>MLESKLKAPVFTATTQGDHYGEFVLEPLERGFGVTLGNPLRRILLSSIPGTAVTSVYIEDVLHEFSTIPGVKEDVVEIILNLKELVVRFLDPKMASTTLILRAEGPKEVRAGDFTPSADVEIMNPDLHIATLEEGGKLYMEVRVDRGVGYVPAERHGIKDRINAIPVDAIFSPVRRVAFQVEDTRLGQRTDLDKLTLRIWTDGSVTPLEALNQAVAILKEHLNYFANPEASLLPTPEVSKGEKRESAEEDLDLPLEELGLSTRVLHSLKEEGIESVRALLALNLKDLRNIPGIGERSLEEIRQALAKKGFTLKE[4x];>MEIKRFGRIREVIPLPPLTEIQVESYKKALQADVPPEKRENVGIQAAFKETFPIEEGDKGKGGLVLDFLEYRIGDPPFSQDECREKDLTYQAPLYARLQLIHKDTGLIKEDEVFLGHLPLMTEDGSFIINGADRVIVSQIHRSPGVYFTPDPARPGRYIASIIPLPKRGPWIDLEVEASGVVTMKVNKRKFPLVLLLRVLGYDQETLVRELSAYGDLVQGLLDEAVLAMRPEEAMVRLFTLLRPGDPPKKDKALAYLFGLLADPKRYDLGEAGRYKAEEKLGVGLSGRTLVRFEDGEFKDEVFLPTLRYLFALTAGVPGHEVDDIDHLGNRRIRTVGELMADQFRVGLARLARGVRERMVMGSPDTLTPAKLVNSRPLEAALREFFSRSQLSQFKDETNPLSSLRHKRRISALGPGGLTRERAGFDVRDVHRTHYGRICPVETPEGANIGLITSLAAYARVDALGFIRTPYRRVKNGVVTEEVVYMTASEEDRYTIAQANTPLEGDRIATDRVVARRRGEPVIVAPEEVEFMDVSPKQVFSLNTNLIPFLEHDDANRALMGSNMQTQAVPLIRAQAPVVMTGLEERVVRDSLAALYAEEDGEVVKVDGTRIAVRYEDGRLVHPLRRYARSNQGTAFDQRPRVRVGQRVKKGDLLADGPASEEGFLALGQNVLVAIMPFDGYNFEDAIVISEELLKRDFYTSIHIERYEIEARDTKLGPERITRDIPHLSEAALRDLDEEGIVRIGAEVKPGDILVGRTSFKGEQEPSPEERLLRSIFGEKARDVKDTSLRVPPGEGGIVVGRLRLRRGDPGVELKPGVREVVRVFVAQKRKLQVGDKLANRHGNKGVVAKILPVEDMPHLPDGTPVDVILNPLGVPSRMNLGQILETHLGLAGYFLGQRYISPVFDGATEPEIKELLAEAFNLYFGKRQGEGFGVDKREKEVLARAEKLGLVSPGKSPEEQLKELFDLGKVVLYDGRTGEPFEGPIVVGQMFIMKLYHMVEDKMHARSTGPYSLITQQPLGGKAQFGGQRFGEMEVWALEAYGAAHTLQEMLTIKSDDIEGRNAAYQAIIKGEDVPEPSVPESFRVLVKELQALALDVQTLDEKDNPVDIFEGLASKR[2x];>MKKEVRKVRIALASPEKIRSWSYGEVEKPETINYRTLKPERDGLFDERIFGPIKDYECACGKYKRQRFEGKVCERCGVEVTRSIVRRYRMGHIELATPAAHIWFVKDVPSKIGTLLDLSATELEQVLYFNKYIVLDPKGAVLDGVPVEKRQLLTDEEYRELRYGKQETYPLPAGVDALVKDGEEVVKGQELAPGVVSRMDGVALYRFPRRVRVDYLRKERAALRIPLSAWVEKEAYRPGEVLAELSEPYLFRAEESGVVELKDLAEGHLIYLRQEEEVVARYFLPAGMTPLVVEGEIVEVGQPLAEGKGLLRLPRHMTAKEVEAEEEGDSVHLTLFLEWTEPKDYKVAPHMNVIVPEGAKVQAGEKIVAAIDPEEEVIAEAEGVVHLHEPASILVVKARVYPFEDDVEVTTGDRVAPGDVLADGGKVKSEIYGRVEVDLVRNVVRVVESYDIDARMGAEAIQELLKELDLEKLERELLEEMKHPSRARRAKARKRLEVVRAFLDSGNRPEWMILEAVPVLPPDLRPMVQVDGGRFATSDLNDLYRRLINRNNRLKKLLAQGAPEIIIRNEKRMLQEAVDAVIDNGRRGSPVTNPGSERPLRSLTDILSGKQGRFRQNLLGKRVDYSGRSVIVVGPQLKLHQCGLPKRMALELFKPFLLKKMEEKAFAPNVKAARRMLERQRDIKDEVWDALEEVIHGKVVLLNRAPTLHRLGIQAFQPVLVEGQSIQLHPLVCEAFNADFDGDQMAVHVPLSSFAQAEARIQMLSAHNLLSPASGEPLAKPSRDIILGLYYITQVRKEKKGAGMAFATPEEALAAYERGEVALNAPIVVAGRETSVGRLKFVFANPDEALLAVAHGLLDLQDVVTVRYLGRRLETSPGRILFARIVGEAVGDEKVAQELIQMDVPQEKNSLKDLVYQAFLRLGMEKTARLLDALKYYGFTLSTTSGITIGIDDAVIPEEKQRYLEEADRKLRQIEQAYEMGFLTDRERYDQVIQLWTETTEKVTQAVFKNFEENYPFNPLYVMAQSGARGNPQQIRQLCGMRGLMQKPSGETFEVPVRSSFREGLTVLEYFISSHGARKGGADTALRTADSGYLTRKLVDVAHEIVVREADCGTTNYISVPLFQMDEVTRTLRLRKRSDIESGLYGRVLAREVEALGRRLEEGRYLSLEDVHFLIKAAEAGEVREVPVRSPLTCQTRYGVCQKCYGYDLSMARPVSIGEAVGVVAAESIGEPGTQLTMRTFHTGGVAVGTDITQGLPRVIELFEARRPKAKAVISEIDGVVRIEEGEDRLSVFVESEGFSKEYKLPKDARLLVKDGDYVEAGQPLTRGAIDPHQLLEAKGPEAVERYLVDEIQKVYRAQGVKLHDKHIEIVVRQMLKYVEVTDPGDSRLLEGQVLEKWDVEALNERLIAEGKVPVAWKPLLMGVTKSALSTKSWLSAASFQNTTHVLTEAAIAGKKDELIGLKENVILGRLIPAGTGSDFVRFTQVVDQRTLKAIEEARKEAVEAKEKEAPRRPVRREQPGKGL[2x];>[2x]MAEPGIDKLFGMVDSKYRLTVVVAKRAQQLLRHRFKNTVLEPEERPKMRTLEGLYDDPNAVTWAMKELLTGRLFFGENLVPEDRLQKEMERLYPTEEEA;>[2x]TSDPVRQYLHEIGQVPLLTLEEEIDLARKVEEGMEAIKKLSEATGLDQELIREVVRAKILGTARVEEVDGKLKSLPKELKRYLHIAREGEAARQHLIEANLRLVVSIAKKYTGRGLSFLDLIQEGNQGLIRAVEKFEYKRRFKFSTYATWWIRQAINRAIADQARTIRIPVHMVETINKLSRTARQLQQELGREPSYEEIAEAMGPGWDAKRVEETLKIAQEPVSLETPIGDEKDSFYGDFIPDENLPSPVEAAAQSLLSEELEKALSKLSEREAMVLKLRKGLIDGREHTLEEVGAYFGVTRERIRQI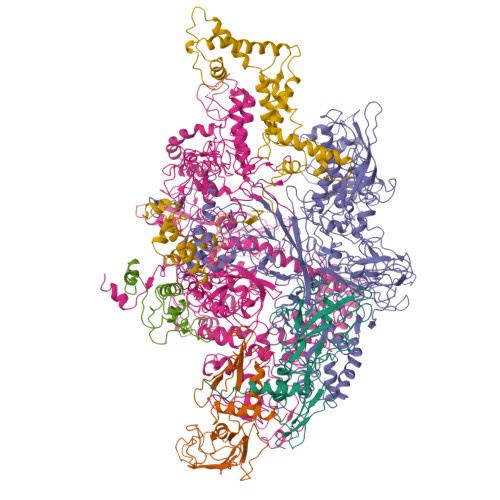ENKALRKLKYHESRTRKLRDFLE>SHEELNDQLRVRREKLKKIEELGVDPFGKRFERTHKAEELFELYGDLSKEELEEQQIEVAVAGRIMTKRGMGKAGFAHIQDVTGQIQIYVRQDDVGEQQYELFKISDLGDIVGVRGTMFKTKVGELSIKVSSYEFLTKALRPLPEKYHGLKDIEQRYRQRYLDLIMNPESKKTFITRSLIIQSMRRYLDSHGYLEVETPMMHAVAGGAAARPFITHHNALDMTLYMRIAIELHLKRLIVGGLEKVYEIGRVFRNEGISTRHNPEFTMLELYEAYADFRDIMKLTENLIAHIATEVLGTTKIQYGEHLVDLTPEWRRLHMVDAIKEYVGVDFWRQMSDEEARELAKEHGVEVAPHMTFGHIVNEFFEQKVEDKLIQPTFIYGHPVEISPLAKKNPDDPRFTDRFELFIVGREHANAFTELNDPIDQRQRFEEQLKEREQGNDEAHEMDEDFLEALEYGMPPTGGLGIGVDRLVMLLTNSPSIRDVLLFPQMRHK[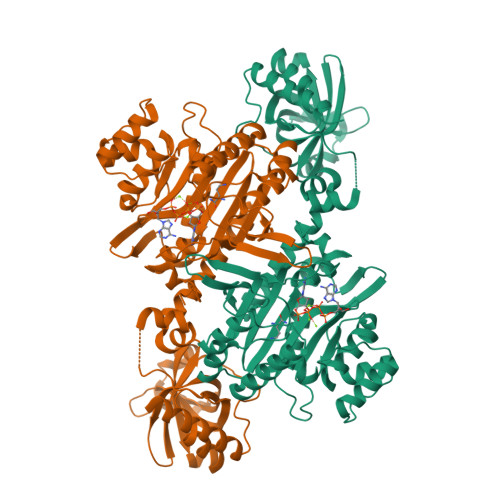4x]> GMTFSLFGDKFTRHSGITRLMEDLNDGLRTPGAIMLGGGNPAHIPAMQDYFQTLLTDMVESGKAADALCNYDGPQGKTALLNALAVLLRETLGWDIEPQNIALTNGSQSAFFYLFNLFAGRRADGSTKKVLFPLAPEYIGYADSGLEDDLFVSARPNIELLPEGQFKYHVDFEHLHIGEETGMICVSRPTNPTGNVITDEELMKLDRLANQHNIPLVIDNAYGVPFPGIIFSEARPLWNPNIILCMSLSKLGLPGSRCGIIIANDKTITAI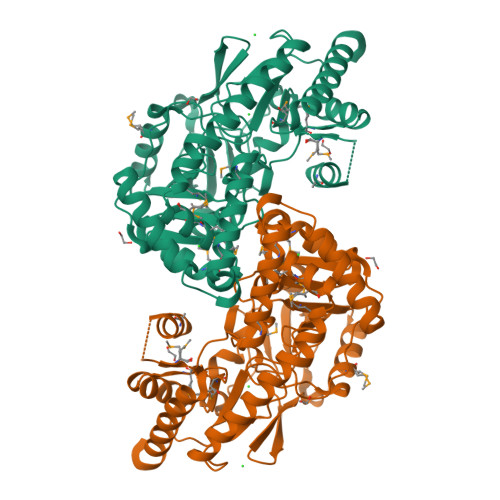ANMNGIISLAPGGMGPAMMCEMIKRNDLLRLSETVIKPFYYQRVQQTIAIIRRYLSEERCLIHKPEGAIFLWLWFKDLPITTELLYQRLKARGVLMVPGHYFFPGLDKPWPHTHQCMRMNYVPEPDKIEAGVKILAEEIERAWREG> MHHHHHHHHGVDLGTENLYFQSNAMLSGKARAHTNIALIKYWGKANEEYILPMNSSLSLTLDAFYTETTVTFDAHYSEDVFILNGILQNEKQTKKVKEFLNLVRQQADCTWFAKVESQNFVPTAAGLASSASGLAALAGACNVALGLNLSAKDLSRLARRGSGSACRSIFGGFAQWNKGHSDETSFAENIPANNWENELAMLFILINDGEKDVSSRDGMKRTVETSSF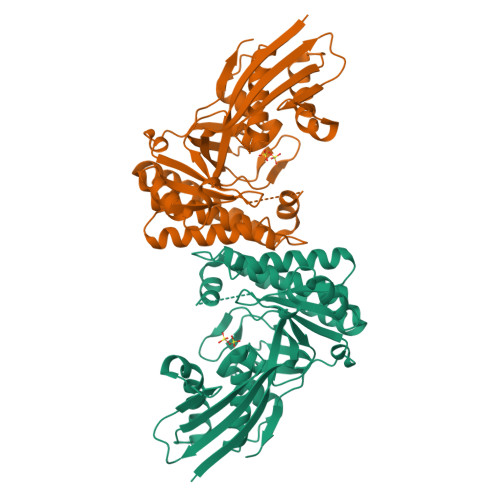YQGWLDNVEKDLSQVHEAIKTKDFPRLGEIIEANGLRMHGTTLGAVPPFTYWSPGSLQAMALVRQARAKGIPCYFTMDAGPNVKVLVEKKNLEALKTFLSEHFSKEQLVPAFAGPGIELFETKGMDK>[2x]GSDQVQKVDQYLYHMRLSDETLLEISKRFRKEMEKGLGATTHPTAAVKMLPTFVRSTPDGTEHGEFLALDLGGTNFRVLWVKVTDNGLQKVEMENQIYAIPEDIMRGSGTQLFDHIAECLANFMDKLQIKDKKLPLGFTFSFPCHQTKLDESFLVSWTKGFKSSGVEGRDVVALIRKAIQRRGDFDIDIVAVVNDTVGTMMTCGYDDHNCEIGLIVGTGSNACYMEEMRHIDMVEGDEGRMCINMEWGAFGDDGSLNDIRTEFDQEIDMGSLNPGKQLFEKMISGMYMGELVRLILVKMAKEELLFGGKLSPELLNTGRFETKDISDIEGEKDGIRKAREVLMRLGLDPTQEDCVATHRICQIVSTRSASLCAATLAAVLQRIKENKGEERLRSTIGVDGSVYKKHPHFAKRLHKTVRRLVPGCDVRFLRSEDGSGKGAAMVTAVAYRLADQHRARQKTLEHLQLSHDQLLEVKRRMKVEMERGLSKETHASAPVKMLPTYVCATPDGTEKGDFLALDLGGTNFRVLLVRVRNGKWGGVEMHNKIYAIPQEVMHGTGDELFDHIVQCIADFLEYMGMKGVSLPLGFTFSFPCQQNSLDESILLKWTKGFKASGCEGEDVVTLLKEAIHRREEFDLDVVAVVNDTVGTMMTCGFEDPHCEVGLIVGTGSNACYMEEMRNVELVEGEEGRMCVNMEWGAFGDNGCLDDFRTEFDVAVDELSLNPGKQRFEKMISGMYLGEIVRNILIDFTKRGLLFRGRISERLKTRGIFETKFLSQIESDCLALLQVRAILQHLGLESTCDDSIIVKEVCTVVARRAAQLCGAGMAAVVDRIRENRGLDALKVTVGVDGTLYKLHPHFAKVMHETVKDLAPKCDVSFLQSEDGSGKGAALITAVACRIREAGQ

Hexokinase, the first enzyme of the glycolytic pathway, catalyzes the irreversible rate-limiting phosphorylation of glucose to glucose-6-phosphate (G6P). The elevated rates of glucose metabolism, tumor progression, and the high patient mortality has been predominantly associated with the overexpression of HK2 in different cancers. HK2 is predominantly co-localized on the outer mitochondrial membrane (OMM), where its translocation is facilitated by an increase in the cellular glucose concentration. The mitochondrial translocation of HK2 not only gives it preferential access to ATP required for its function and relieves feedback inhibition by G6P, but most importantly, suppresses apoptosis.

For in vitro biochemical characterization of the mitochondrial conformation, a variant lacking the MBP, the first 16 amino acids of the N-terminus (Δ16), will mimic the HK2 conformation on the mitochondria. Only the Δ16 variant of the WT-HK2 crystallized in complex with glucose and G6P at 2.45 Å. The crystal structure of human HK2 is a homodimer with two structurally identical N- and C-halves of equal size linked by a long eight-turn linker helix-α13. Similar to the overall fold of mammalian hexokinases, the N- and C-domains have an identical α/β fold that is conserved amongst the hexokinase family. Each domain is distinctly folded into large and small subdomains that each contains a five stranded mixed β-sheet. The active site is formed by a cleft between the two subdomains, where their β-sheets enclose the active site and the helices α5 and α13. The N-half of HK2 is linked to the C-half by helix-α13 that protrudes out of the active site of the N-domain. Helix-α5 that is perpendicular to the linker helix-α13, carries the catalytic residue D209 of the N-half. The glucose-binding pockets in the N- and C-halves of HK2 are identical to other members of the hexokinase family, with the requirement of an aspartic residue for catalysis. The catalytic residue D209 or D657 of the N- and C-domains, respectively, forms H-bonding interactions with the 4-OH and 6-OH of glucose, and a lysine residue, K173 or K621, align the γ-phosphate of ATP with the 6-OH of glucose for its phosphorylation.>GHMTLPTKTSTLDVAAQCFLNSLVRETKDWRLTEYQPTQLIIPLGEQQALHFRVAYFSPTQHHRFEFPARLVTASGSHPVDFATLSRLIVDKLQHQLLLPATSCETFHQRVMESHAHTQQAIDARHDWAALREKALNFGEAEQALLVGHAFHPAPKSHEPFNQQEAERYLPDFAPHFPLRWFAVNKTQIAGESLHLNLQQRLTRFAAENAPQLLNELSDNQWLFPLHPWQGEYLLQQEWCQELVAKGLIKDLGEAGAPWLPTTSSRSLYCATSRDMIKFSLSVRLTNSVRTLSVKEVKRGMRLARLAQTDDWQTLQARFPTFRVMQEDGWAGLRDLHGNIMQESLFALRENLLVDQPQSQTNVLVSLTQAAPDGGDSLLVAAVKRLSDRLGITAQQAAHAWVDAYCHQVLKPLFTAEADYGLVLLAHQQNILVQMLGDLPVGLIYRDCQGSAFMPHA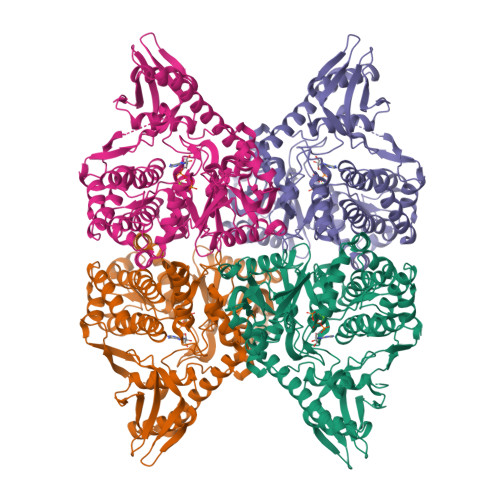AGWLDTIGEAQAENVFTREQLLRYFPYYLLVNSTFAVTAALGAAGLDSEANLMARVRTLLAEMRDQVTHKTCLNYVLENPYWNVKGNFFCYLNDHNENTIVDPSVIYFDFANPLLAQEG[8x]> MGSSHHHHHHSSGRENLYFQGMYNTISITVVDADDVGVNFVVSKVLSTLHNKGIFNGEVGVTFPRMDKNVGDIITLFSKTGVDRKVLTSTLNTLTDFIHIGKPKEADKVKTYRKVDT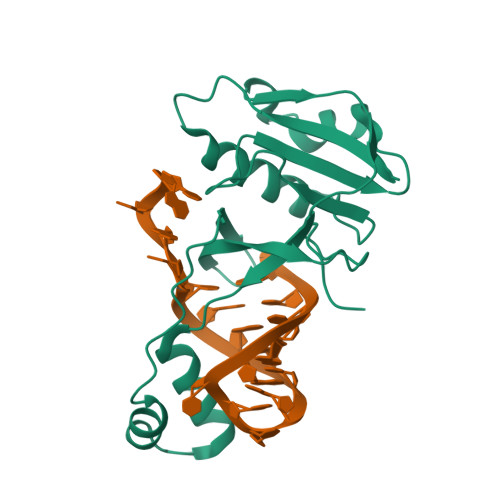KSKGKLIRRCIKRKGVSAETAESLYGNYKGEKCKLPYIVVNSKSTGQRFSMFLEECENSEKFNSYGLCIVSC>[2x]MPHFTVTKVEDPEEGAAASISQEPSLADIKARIQDSDEPDLSQNSITGEHSQLLDDGHKKARNAYLNNSNYEEGDEYFDKNLALFEEEMDTRPKVSSLLNRMANYTNLTQGAKEHEEAENITEGKKKPTKTPQMGTFMGVYLPCLQNIFGVILFLRLTWVVGTAGVLQAFAIVLICCCCTMLTAISMSAIATNGVVPAGGSYFMISRALGPEFGGAVGLCFYLGTTFAAAMYILGAIEIFLVYIVPRAAIFHSDDALKESAAMLNNMRVYGTAFLVLMVLVVFIGVRYVNKFASLFLACVIVSILAIYAGAIKSSFAPPHFPVCMLGNRTLSSRHIDVCSKTKEINNMTVPSKLWGFFCNSSQFFNATCDEYFVHNNVTSIQGIPGLASGIITENLWSNYLPKGEIIEKPSAKSSDVLGSLNHEYVLVDITTSFTLLVGIFFPSVTGIMAGSNRSGDLKDAQKSIPIGTILAILTTSFVYLSNVVLFGACIEGVVLRDKFGDAVKGNLVVGTLSWPSPWVIVIGSFFSTCGAGLQSLTGAPRLLQAIAKDNIIPFLRVFGHSKANGEPTWALLLTAAIAELGILIASLDLVAPILSMFFLMCYLFVNLACALQTLLRTPNWRPRFRYYHWALSFMGMSICLALMFISSWYYAIVAMVIAGMIYKYIEYQGAEKEWGDGIRGLSLSAARFALLRLEEGPPHTKNWRPQLLVLLKLDEDLHVKHPRLLTFASQLKAGKGLTIVGSVIVGNFLENYGEALAAEQTIKHLMEAEKVKGFCQLVVAAKLREGISHLIQSCGLGGMKHNTVVMGWPNGWRQSEDARAWKTFIGTVRVTTAAHLALLVAKNISFFPSNVEQFSEGNIDVWWIVHDGGMLMLLPFLLKQHKVWRKCSIRIFTVAQLEDNSIQMKKDLATFLYHLRIEAEVEVVEMHDSDISAYTYERTLMMEQRSQMLRHMRLSKT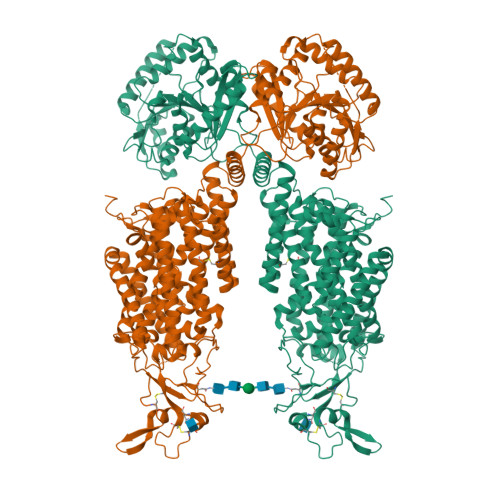ERDREAQLVKDRNSMLRLTSIGSDEDEETETYQEKVHMTWTKDKYMASRGQKAKSMEGFQDLLNMRPDQSNVRRMHTAVKLNEVIVNKSHEAKLVLLNMPGPPRNPEGDENYMEFLEVLTEGLERVLLVRGGGSEVITIYS During biosynthesis by multi-modular trans-AT polyketide synthases, polyketide structural space can be expanded by conversion of initially-formed electrophilic β-ketones into β-alkyl groups. These multi-step transformations are catalysed by 3-hydroxy-3-methylgluratryl synthase cassettes of enzymes. In this work, we investigated the β-methylation module 5 present in the virginiamycin (Vir) trans-AT PKS-NRPS, which comprises a KS domain and tandem ACPs (ACP5a and ACP5b). We show here that β-methylation cassette members VirC, VirD and VirE do indeed preferentially recognise ACP5b, even when the ACP is excised from its modular context, and that β-modification occurs within defined ACP5b/partner complexes.

Instead, the crystal structure of the holo-ACP5b–VirD complex identifies an ACP interaction motif centred on the phosphopantetheine (Ppant) prosthetic arm and surrounding secondary structural elements, with specificity conferred via distinctive electrostatic surface features of the domain combined with precise Ppant positioning. As evidenced by the H3 crystal symmetry, VirD forms characteristic homotrimeric disks, two of which are stacked, with six ACPs distributed equatorially at the interface between the trimers. In this arrangement, the smallest gap between S6871 of ACP5b bearing the Ppant (∼20 Å) and the catalytic E128 of a VirD monomer is ca. 13.9 Å, with the other VirD active sites more than 33.8 Å distant. VirD elements contributing to the interface include the β-strand β10 and the subsequent loop (β10–α4) of one monomer, and the β-turn (β1–β2), the loop (α1–β4) and helix α7 of a second monomer. Notably, the interface also incorporates the well-folded helix α10 of the first monomer, which is disordered in the structure of VirD alone. Concerning the ACP, the interaction involves the C-terminal portion of helix α1, the adjacent loop (α1–α2) and the N-terminal regions of helices α2 and α3. The structure of the complex also identifies key interactions between VirD and the Ppant tethered to S6871 of ACP5b (the distal end of which is not visible in the electron density), consistent with its contribution to binding affinity as observed by fluorescence quenching. Specifically, R125 of VirD, whose side chain is oriented by a water molecule, forms a salt bridge with the Ppant phosphate. The same water molecule bridges R192 from an adjacent VirD monomer, which participates in a salt bridge with D6870 of ACP5b. Gratifyingly, close inspection of the holo-ACP5b–VirD complex structure identified ACP5b N6865 located in the α1–α2 loop as a potential specificity determinant.

>GPGSVRVVRGRGLLRAVLDRPERRNPIDAGLLTSLARALDQAESDQDCRVFVLSSTGEDFCAGTDLSGGDPAPEPLPDGAELPYWTLLERLTRSPLATVAVVDGRATAGGVGLAAACDLVLAGERARFRLTEVLAGLVPAMALPFVARRTGEQRAFAATLRAEEFDAGAAHRVGLADLAGPRAEDLLPPVLAGLGRTDRSTTAALKEYRARLFPRDARLGHDASRLLIERFAAPGTGQLLARLREAGAAA[2x];>[2x]GPGSAVAVDPAPVARALREELARTLYCEPGDIDDEASFNTLGLDSILGVEFVAFVNQTYGLDEKAGILYDHPSLAALSRHVAGRAAPV3-(2-methylphenyl)benzoic acid | C14 H12 O2 | 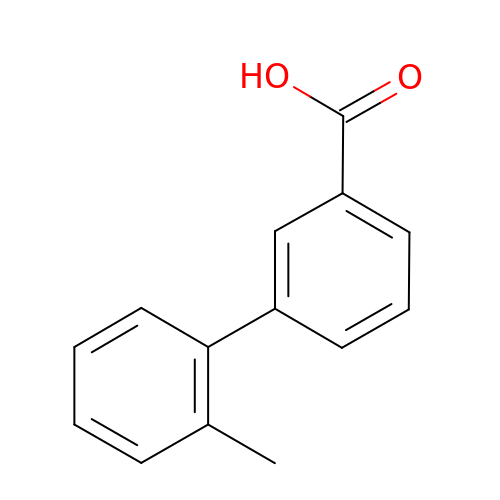IAZJDWZUCUHVPQ-UHFFFAOYSA-N>XYRIPSYDFADELAKLLRQAA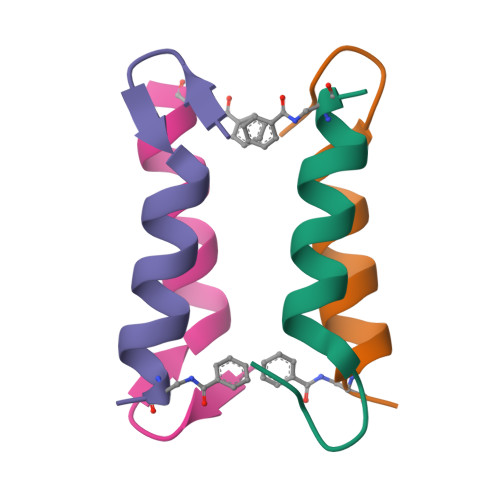GX[4x]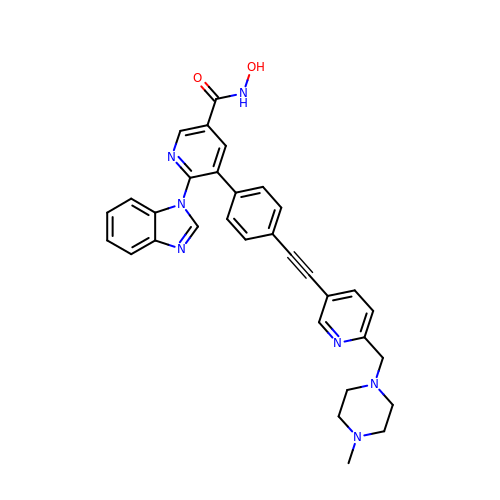6-(1H-benzimidazol-1-yl)-N-hydroxy-5-[4-({6-[(4-methylpiperazin-1-yl)methyl]pyridin-3-yl}ethynyl)phenyl]pyridine-3-carboxamide | C32 H29 N7 O2 | YJCPLYNHCKYCMY-UHFFFAOYSA-N> MGAHASVIKPEMKIKLRME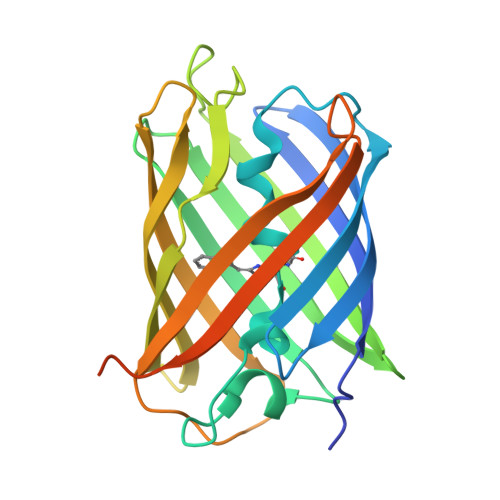GAVNGHKFVIEGEGIGKPYEGTQTLDLTVEEGAPLPFSYDILTPAFQWGNRAFTKYPEDIPDYFKQAFPEGYSWERSMTYEDQGICIATSDITMEGDCFFYEIRFDGTNFPPNGPVMQKKTLKWEPSTEKMYVEDGVLKGDVEMALLLEGGGHYRCDFKTTYKAKKDVRLPDAHEVDHRTEILSHDKDYNKVRLYEHAEARYSGGGSGGGASGKPIPNPLLGLDSTHHHHHH>[2x]MPATDTLSLSASEALARRRSVRAFTDRPVDRALLARIFEIAQRAPSGGNLQPWQATVVTGERWQAVQDAVAARIVMGREGFQPEYDIFPRGLTDPWD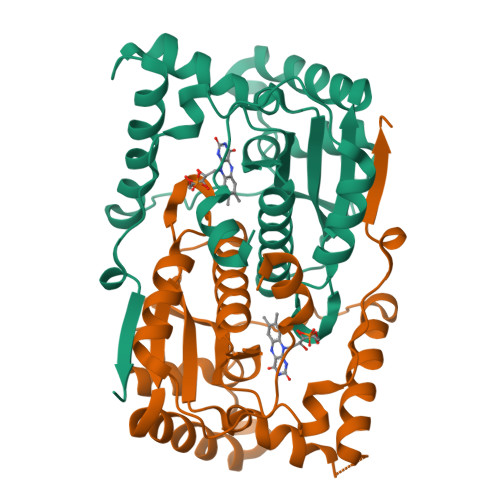SRRFGVGEALYASLGIARDDKAGRIAQFQQNYRGFGAPVMLFLHCSRIMGPPQWADMGMWLQSVMLLLVEHGLASCPQECWAMYGATVRAELGLGDDQILFSGLAIGHADEEAPVNRWPVPRVGLDEVIDWQGFDA(1P)-N-(5-tert-butyl-2-{[(3R)-hexan-3-yl]oxy}phenyl)-1-(2,5-dimethoxyphenyl)-5-methyl-1H-1,2,3-triazole-4-carboxamide 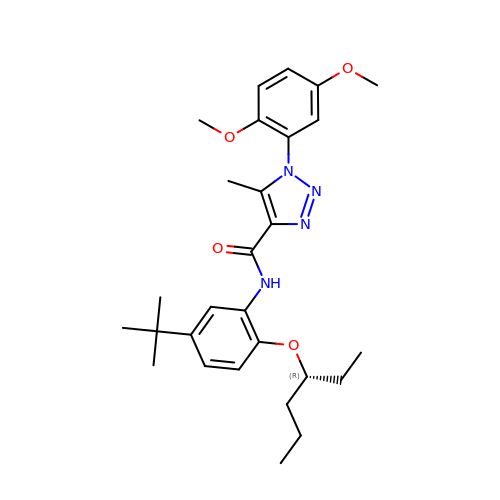| C28 H38 N4 O4 | HPFQSDGKIYUBEE-HXUWFJFHSA-N>MQVHVIRRENRALYAGLLEKYFRIRHQIYVVERGWKELDRPDGREIDQFDTEDAVYLLGVDNDDIVAGMRMVPTTSPTLLSDVFPQLALAGPVRRPDAYELSRIFVVPRKRGEHGGPRAEAVIQAAAMEYGLSIGLSAFTIVLETWWLPRLVDQGWKAKPLGLPQDINGFSTTAVIVDVDDDAWVGICNRRSVPGPTLEWRGLEAIRRHS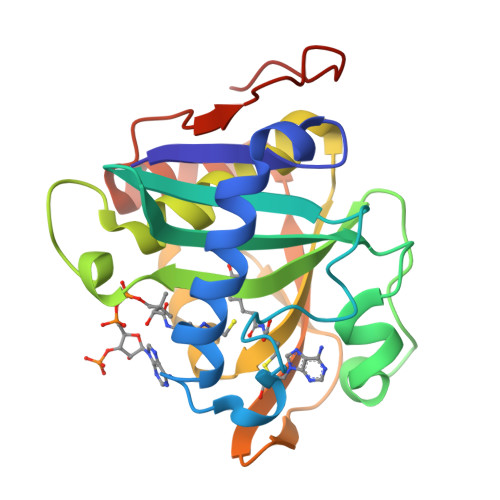LPE[2x]>SDKPKRPLSA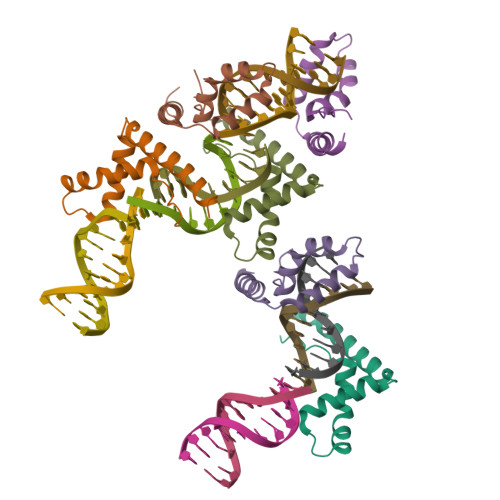YALWLNSARESIKRENPGIKVTEVAKRGGELWRAMKDKSEWEAKAAKAKDDYDRAVKEFEANG[6x]> SGIRELNLTKEQHEWLNGWLELWGAWVYSGRLEKRMSSVIAKFMESVEPGRVMTRPMCNDDDGMLISQVVDSVMYIDKKAFGILLSYYAHGSSKH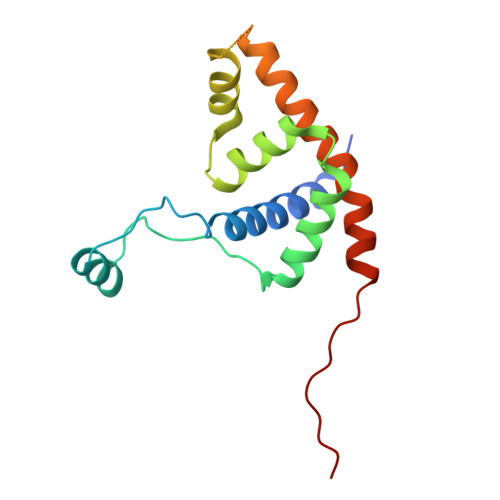AIASYYHRVARPRKMLCRGGGRIQKPSLATCRREVDEILNASLFMIYPVLDSAFKNRKRVEKIKHVA>[2x]GPGSHLAHPNLDTFTPEELLQQMKELLTKNHQLKEAMKLNNQAMKGRFEELSAWTEKQ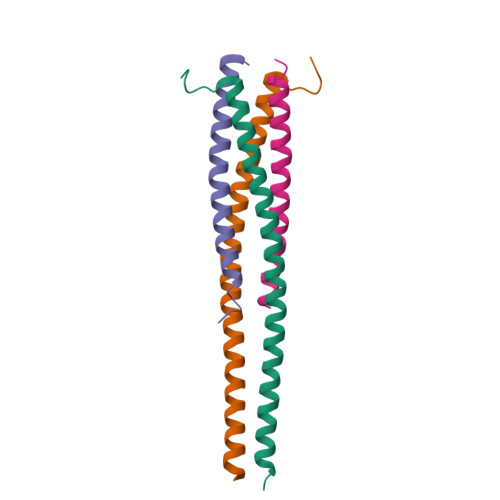KEERQFFEIQSKEAKERLMALSHE;>GPGSYPSSNTLVEMTLGMKKLKEEMEGVVKELAENNHILERFGSLTMDGGLRNVDCL[2x]>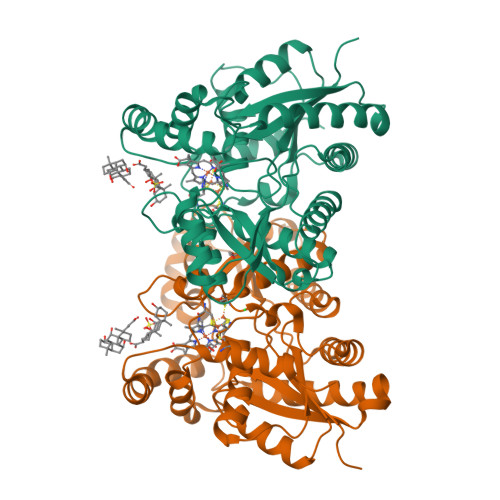[2x]RKPKTGILMLNMGGPETLGDVHDFLLRLFLDRDLMTLPIQNKLAPFIAKRRTPKIQEQYRRIGGGSPIKIWTSKQGEGMVKLLDELSPNTAPHKYYIGFRYVHPLTEEAIEEMERDGLERAIAFTQYPQYSCSTTGSSLNAIYRYYNQVGRKPTMKWSTIDRWPTHHLLIQCFADHILKELDHFPLEKRSEVVILFSAHSLPMSVVNRGDPYPQEVSATVQKVMERLEYCNPYRLVWQSKVGPMPWLGPQTDESIKGLCERGRKNILLVPIAFTSDHIETLYELDIEYSQVLAKECGVENIRRAESLNGNPLFSKALADLVHSHIQSNELCSKQLTLSCPLCVNPVCRETKSFFTSQQL> MASMTGGQQMGRDEAGITGTWYNQLGSTFIVTAGADGALTGTYESAAGKAESRYVLTGRYDSAPATDGSGTALGWTVAWKNNYRNAHSATTWSGQYVGGAEARINTQWLLTSGQTEANGWRSTLVGHDTFTKVKPSAASIDAAKKAGVNNGNPLDAVQQ

We describe here the use of an artificial cofactor employing the well‐known biotin‐streptavidin system to catalyze a Baylis‐Hillman reaction. As protein host, we chose streptavidin, as it can be easily crystallized and thereby supports the design process. There are several examples using streptavidin as the host for these cofactors, since its natural ligand biotin binds strongly (K d∼10−15 M) and is easy to modify with catalysts at the carboxylic acid group. No enzyme is known to naturally catalyze the Baylis‐Hillman reaction, a very versatile and atom‐economic C−C bond forming reaction for the production of various functionalized compounds and intermediates of active pharmaceutical ingredients (APIs).

We chose a derivative of DMAP as the artificial cofactor due to its low steric demand, which will facilitate its inclusion into the protein scaffold. The protein host around the cofactor was rationally designed on the basis of high‐resolution crystal structures obtained after each variation of the amino acid sequence. The location of the catalyst is in a shallow cavity at the surface of the protein. The system was evolved through repeated cycles of mutagenesis, activity tests, and structure determination. According to the presented structures and calculations the catalytically active site is too shallow to undergo interactions with 1.>MSSSNVEVFIPVSQGNTNGFPATASNDLKAFTEGAVLSFHNICYRVKLKSGFLPCRKPVEKEILSNINGIMKPGLNAILGPTGGGKSSLLDVLAARKDPSGLSGDVLINGAPRPANFKCNSGYVVQDDVVMGTLTVRENLQFSAALRLATTMTNHEKNERINRVIQELGLDKVADSKVGTQFIRGVSGGERKRTSIGMELITDPSILFLDEPTTGLDSSTANAVLLLLKRMSKQGRTIIFSIHQPRYSIFKLFDSLTLLASGRLMFHGPAQEALGYFESAGYHCEAYNNPADFFLDIINGDSTAVALNREEDFKATEIIEPSKQDKPLIEKLAEIYVNSSFYKETKAELHQLSGGEKKKKITVFKEISYTTSFCHQLRWVSKRSFKNLLGNPQASIAQIIVTVVLGLVIGAIYFGLKNDSTGIQNRAGVLFFLTTNQCFSSVSAVELFVVEKKLFIHEYISGYYRVSSYFLGKLLSDLLPMRMLPSIIFTCIVYFML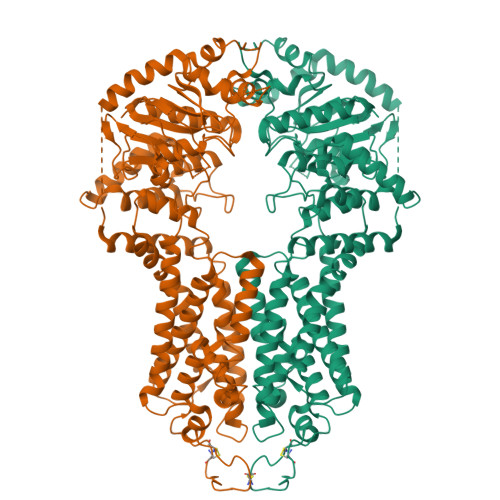GLKPKADAFFVMMFTLMMVAYSASSMALAIAAGQSVVSVATLLMTICFVFMMIFSGLLVNLTTIASWLSWLQYFSIPRYGFTALQHNEFLGQNFCPGLNATGNNPCNYATCTGEEYLVKQGIDLSPWGLWKNHVALACMIVIFLTIAYLKLLFLKKYS[2x]N-(3-fluoro-4-{[1-methyl-6-(1H-pyrazol-4-yl)-1H-indazol-5-yl]oxy}phenyl)-1-(4-fluorophenyl)-6-methyl-2-oxo-1,2-dihydropyridine-3-carboxamide | C30 H22 F2 N6 O3 | 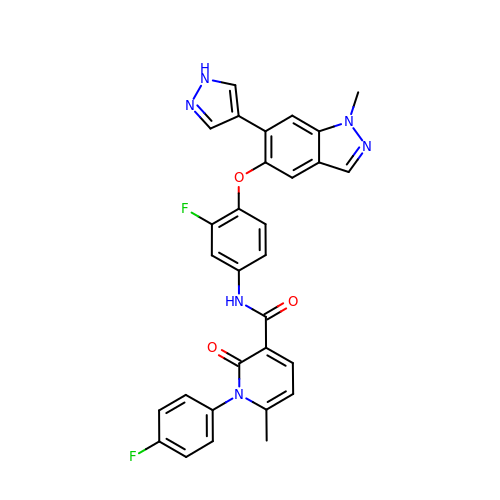QHADVLVFMKEIIP-UHFFFAOYSA-N> MRVNNGLTPQELEAYGISDVHDIVYNPSYDLLYQEELDPSLTGYERGVLTNLGAVAVDTGIFTGRSPKDKYIVRDDTTRDTFWWADKGKGKNDNKPLSPETWQHLKGLVTRQLSGKRLFVVDAFCGANPDTRLSVRFITEVAWQAHFVKNMFIRPSDE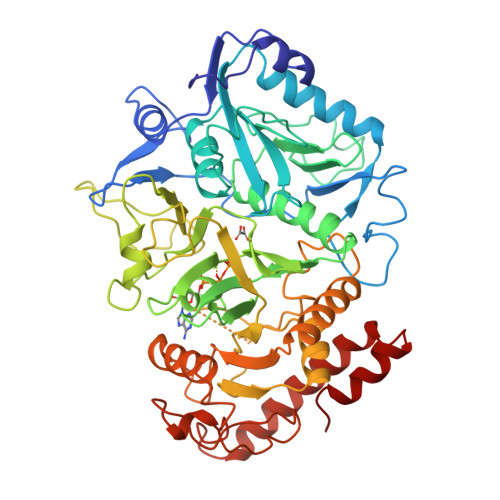ELAGFKPDFIVMNGAKCTNPQWKEQGLNSENFVAFNLTERMQLIGGTWYGGEMKKGMFSMMNYLLPLKGIASMHCSANVGEKGDVAVFFGLSGTGKTTLSTDPKRRLIGDDEHGWDDDGVFNFEGGCYAKTIKLSKEAEPEIYNAIRRDALLENVTVREDGTIDFDDGSKTENTRVSYPIYHIDNIVKPVSKAGHATKVIFLTADAFGVLPPVSRLTADQTQYHFLSGFTAKLAGTERGITEPTPTFSACFGAAFLSLHPTQYAEVLVKRMQAAGAQAYLVNTGWNGTGKRISIKDTRAIIDAILNGSLDNAETFTLPMFNLAIPTELPGVDTKILDPRNTYASPEQWQEKAETLAKLFIDNFDKYTDTPAGAALVAAGPKLS> GUACG;> CG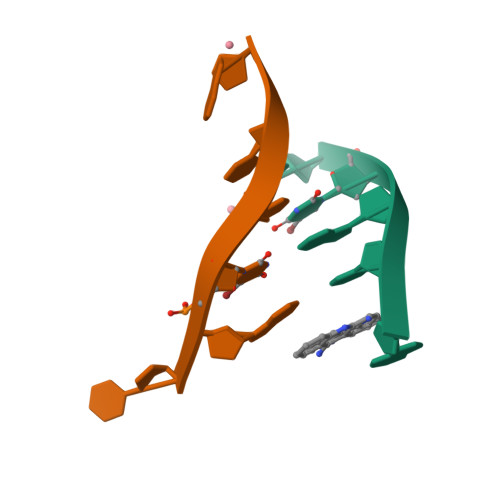UACG>MDEFEMIKRNTSEIISEEELREVLKKDEKSARIGFEPSGKIHLGHYLQIKKMIDLQNAGFDIIIYLADLGAYLNQKGELDEIRKIGDYNKKVFEAMGLKAKYVYGSENCLDKDYTLNVYRLALKTTLKRARRSMELIAREDENPKVAEVIYPIMQVNNIHYSGVDVAVGGMEQRKIHMLARELLPKKVVCIHNPVLTGLDGEGKMSSSKGNFIAVDDSPEEIRAKIKKAYCPAGVVEGNPIMEIAKYFLEYPLTIKRPEKFGGDLTVNSYEELESLFKNKELHPMDLKNAVAEELIKILEPIRKRLLEHHHHHH[2x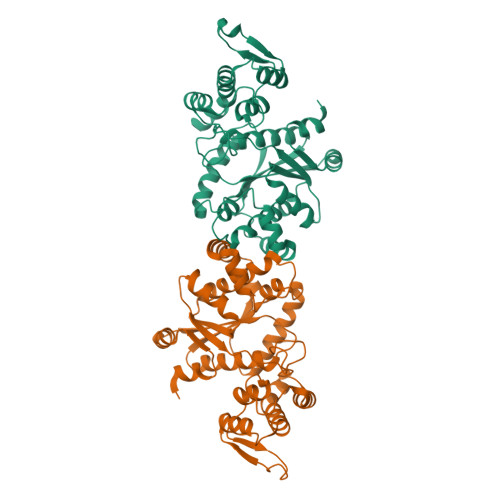]>MSKSDVFHLGLTKNDLQGATLAIVPGDPDRVEKIAALMDKPVKLASHREFTTWRAELDGKPVIVCSTGIGGPSTSIAVEELAQLGIRTFLRIGTTGAIQPHINVGDVLVTTASVRLDGASLHFAPLEFPAVADFECTTALVE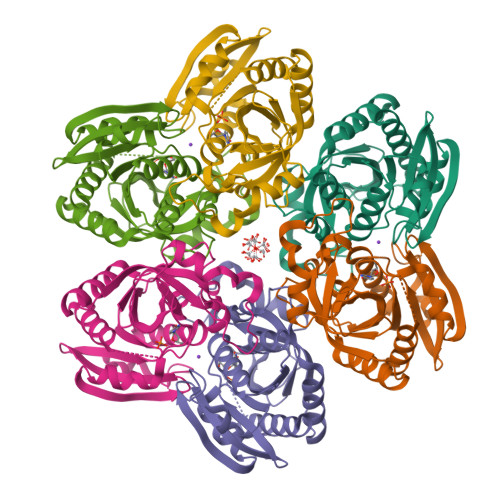AAKSIGATTHVGVTASSDTFYPGQERYDTYSGRVVRHFKGSMEEWQAMGVMNYEMESATLLTMCASQGLRAGMVAGVIVNRTQQEIPNAETMKQTESHAVKIVVEAARRLL[30x]> GAMASTEKRLLKEYRAVKKELTEKRSPIHDTGIV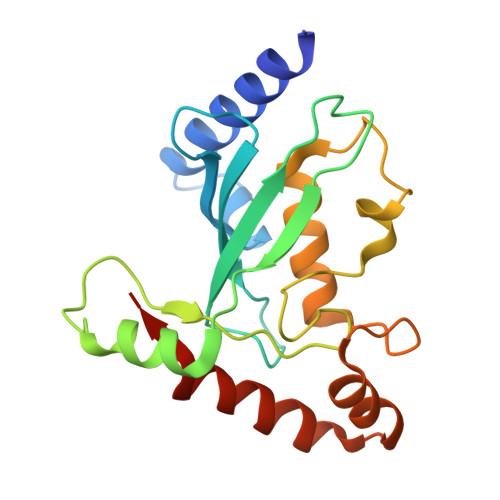DLHPLEDGLFRWSAVIRGPDQSPFEDALWKLEIDIPTNYPLDPPKIKFVVFGEEKIRQLQRKTSSGARKVCYKMPHPNVNFKTGEICLDILQQKWSPAWTLQSALVAIVVLLANPEPLSPLNIDMANLLKCDDTTAYKDLVHYYIAKYSAYESNDV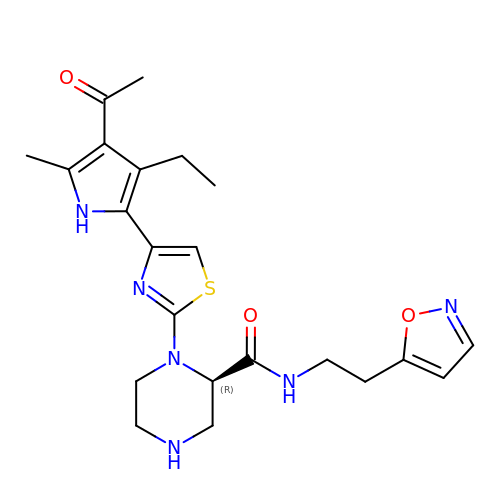(2R)-1-[4-(4-ethanoyl-3-ethyl-5-methyl-1H-pyrrol-2-yl)-1,3-thiazol-2-yl]-N-[2-(1,2-oxazol-5-yl)ethyl]piperazine-2-carboxamide | C22 H28 N6 O3 S | MGZJHFUJKNWRTF-GOSISDBHSA-N D-ARGININE | C6 H15 N4 O2 | 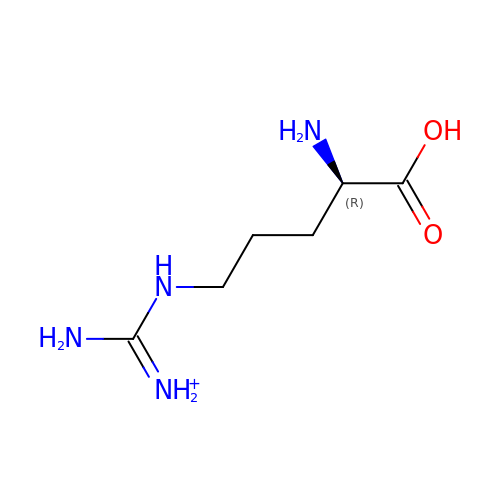ODKSFYDXXFIFQN-SCSAIBSYSA-O4-amino-N-(4-chlorobenzyl)-1,2,5-oxadiazole-3-carboxamide | C10 H9 Cl N4 O2 | 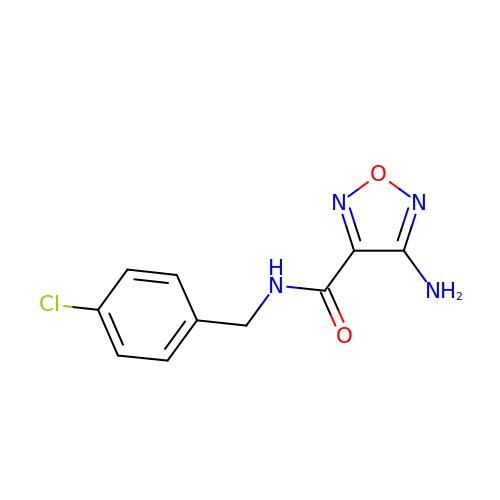WIWIWZDRJHCWJZ-UHFFFAOYSA-N>GANRTLIVTTILEEPYVMYRKSDKPLYGNDRFEGYCLDLLKELSNILGFLYDVKLVPDGKYGAQNDKGEWNGMVKELIDHRADLAVAPLTITYVREKVIDFSKPFMTLGISILYRKGTPIDSADDLAKQ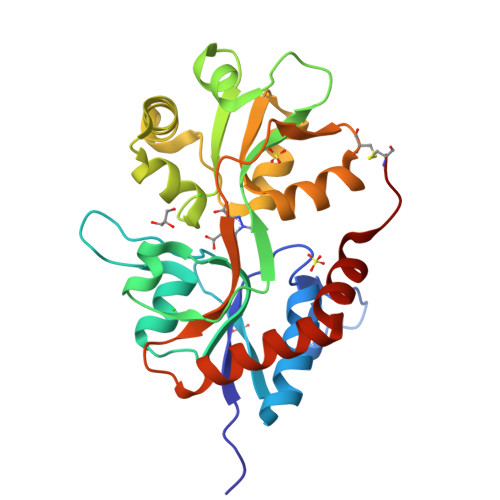TKIEYGAVRDGSTMTFFKKSKISTYEKMWAFMSSRQQSALVKNSDEGIQRVLTTDYALLMESTSIEYVTQRNCNLTQIGGLIDSKGYGVGTPIGSPYRDKITIAILQLQEEGKLHMMKEKWWRGNGCP[2x]>[2x]SNAMATQD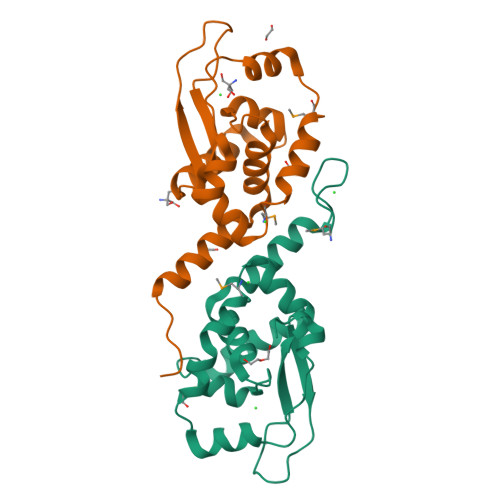RGERPNGFGDELERRRFVLHETRLDVLHQILAQPDGVLSVEELLYRNPDETEANLRYHVDELVDRGIVEKIPVPRAKSVDDPPTTFYAVTGEGIALLRAVSMYEEAAVWRSVYEQMERTDRIEAIENLETRPDVDYESRGATA> EGSITQGTPLKY;> FTTGLVYDTLMLKHQCTCGSSSSHPEHAGRIQSIWSRLQETGLRGKCECIRGRKATLEELQTVHSEAHTLLYGTNPLNRQKLDSKKLLGSLASVFVRLPCGGVGVDSDTIWNEVHSAGAARLAVGCVVELVFKVATGELKNGFAVVRPPGHHAEESTPMGFCYFNSVAVAAKLL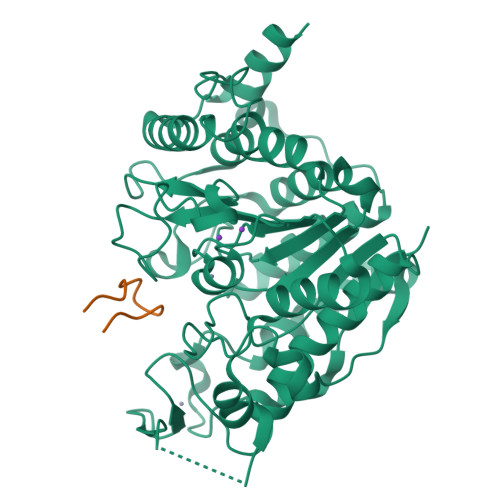QQRLSVSKILIVDWDVHHGNGTQQAFYSDPSVLYMSLHRYDDGNFFPGSGAPDEVGTGPGVGFNVNMAFTGGLDPPMGDAEYLAAFRTVVMPIASEFAPDVVLVSSGFDAVEGHPTPLGGYNLSARCFGYLTKQLMGLAGGRIVLALEGGYDLTAICDASEACVSALLGNELDPLPEKVLQQRPNANAVRSMEKVMEIHSKYWRCLQRTTSTAGRSLIEAQTCEN>MRCVGVGNRDFVEGLSGATWVDVVLEHGGCVTTMAKNKPTLDIELQKTEATQLATLRKLCIEGKITNITTDSRCPTQGEAILPEEQDQNYVCKHTYVDRGWGNGCGLFGKGSLVTCAKFQCLESIEGKVVQHENLKYTVIITVHTGDQHQVGNETQGVTAEITSQASTAEAILPEYGTLGLECSPRTGLDFNEMILLTMKNKAWMVHRQWFFDLPLPWTSGATTKTPTWNRKELLVTFKNAHAKKQEVVVLGSQEGAMHTALTGATEIQTSGGTSIFAGHLKCRLKMDKLKLKGMSYAMCLNTFVLKKEVSETQHGTILIKVEYKGEDAPCKIPFSTEDGQGKAHNGRLITANPVVTKKEEPVNIEAEPPFGESNIVIGIGDKALKINWYRKGF[3x]

The human monoclonal antibody C10 exhibits extraordinary cross-reactivity, potently neutralizing Zika virus (ZIKV) and the four serotypes of dengue virus (DENV1–DENV4). Here we describe a comparative structure-function analysis of C10 bound to the envelope (E) protein dimers of the five viruses it neutralizes. The neutralizing antibodies induced during a DENV or ZIKV infection target the envelope (E) protein and, with a few exceptions, are serotype specific. The epitopes are distributed evenly at the surface of the icosahedral virion, which is composed of 90 E dimers organized in 30 “rafts” of three parallel E dimers (Kuhn et al., 2002).

The kl hairpin adopts variable conformations, being also often disordered in structures of unbound sE, which relate to the curvature of the sE dimers in each structure.>[4x]SIPETQKGVIFYESHGKLEYKDIPVPKPKANELLINVKYSGVCHTDLHAWHGDWPLPTKLPLVGGHEGAGVVVGMGENVKGWKIGDYAGIKWLNGSCMACEYCELGNESNCPHADLSGYTHDGSFQEYATADAVQAAHIPQGTDLAEVAPVLCAGIT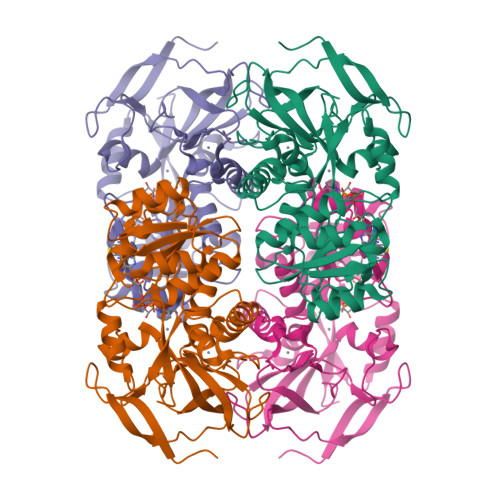VYKALKSANLMAGHWVAISGAAGGLGSLAVQYAKAMGYRVLGIDGGEGKEELFRSIGGEVFIDFTKEKDIVGAVLKATDGGAHGVINVSVSEAAIEASTRYVRANGTTVLVGMPAGAKCCSDVFNQVVKSISIVGSYVGNRADTREALDFFARGLVKSPIKVVGLSTLPEIYEKMEKGQIVGRYVVDTSK non-oxidative branch of the PPP, has been identified in M. TKT enzyme (Rv1449) can convert sedoheptulose-7-phosphate to D-ribose-5-phosphate. mass of 70–75 kDa, with the homodimer being the active entity. The reaction proceeds via a Ping Pong Bi Bi mechanism.

mycobacterial species have not yet been reported. Given the potential importance of TKT in the production of arabinan in M. Recombinant TBTKT was purified in three steps. and purified further using size exclusion chromatography. 2 mM TPP, 5 mM β-mercaptoethanol (pH 7.4). model, built using Swiss-Model and the TKT structure from E. corresponds to amino acids 490–507 in this enzyme.

>MTTLEEISALTRPRHPDYWTEIDSAAVDTIRVLAADAVQKVGNGHPGTAMSLAPLAYTLFQRTMRHDPSDTHWLGRDRFVLSAGHSSLTLYIQLYLGGFGLELSDIESLRTWGSKTPGHPEFRHTPGVEITTGPLGQGLASAVGMAMASRYERGLFDPDAEPGASPFDHYIYVIASDGDIEEGVTSEASSLAAVQQLGNLIVFYDRNQISIEDDTNIALCEDTAARYRAYGWHVQEVEGGENVVGIEEAIANAQAVTDRPSFIALRTVIGYPAPNLMDTGKAHGAALGDDEVAAVKKIVGFDPDKTFQVREDVLTHTRGLVARGKQAHERWQLEFDAWARREPERKALLDRLLAQKLPDGWDADLPHWEPGSKALATRAASGAVLSALGPKLPELWGGSADLAGSNNTTIKGADSFGPPSISTKEYTAHWYGRTLHFGVREHAMGAILSGIVLHGPTRAYGGTFLQFSDYMRPAVRLAALMDIDTIYVWTHDSIGLGEDGPTHQPIEHLSALRAIPRLSVVRPADANETAYAWRTILARRNGSGPVGLILTRQGVPVLDGTDAEGVARGGYVLSDAGGLQPGEEPDVILIATGSEVQLAVAAQTLLADNDILARVVSMPCLEWFEAQPYEYRDAVLPPTVSARVAVEAGVAQCWHQLVGDTGEIVSIEHYGESADHKTLFREYGFTAEAVAAAAERALDN[4x]> MGSSHHHHHHSQDPEQSTPDEVNAALD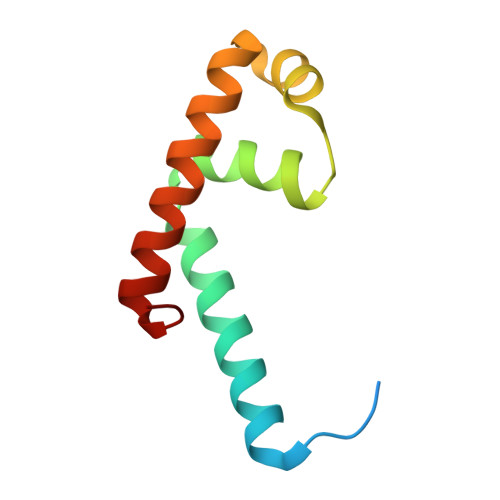RLLIADALAQLSAEHRAVIQRSYYRGWSTAQIATDLGIAEGTVKSRLHYAVRALRLTLQELGVTR>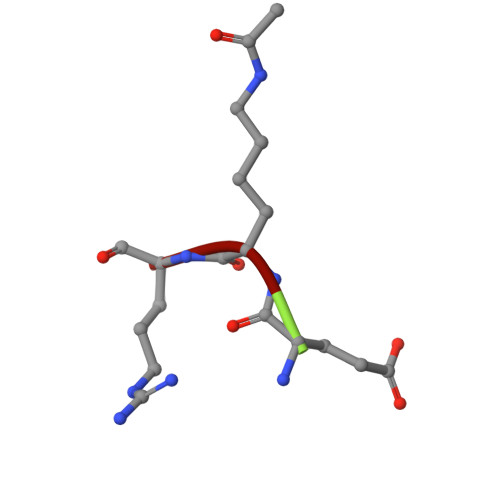 EKR>[4x]GSHMTDLNIPHTHAHLVDAFQALGIRAGQALMLHASVKAVGAVMGGPNVILQALMDALTPDGTLMMYAGWQDIPDFIDSLPDALKAVYLEQHPPFDPATARAVRENSVLAEFLRTWPCVHRSANPEASMVAVGRQAALLTANHALDYGYGVESPLAKLVAIEGYV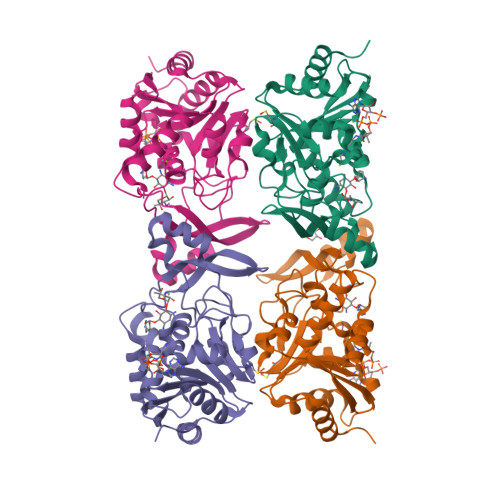LMLGAPLDTITLLHHAEYLAKMRHKNVVRYPCPILRDGRKVWVTVEDYDTGDPHDDYSFEQIARDYVAQGGGTRGKVGDADAYLFAAQDLTRFAVQWLESRFGDSASYG ROLIPRAM | C16 H21 N O3 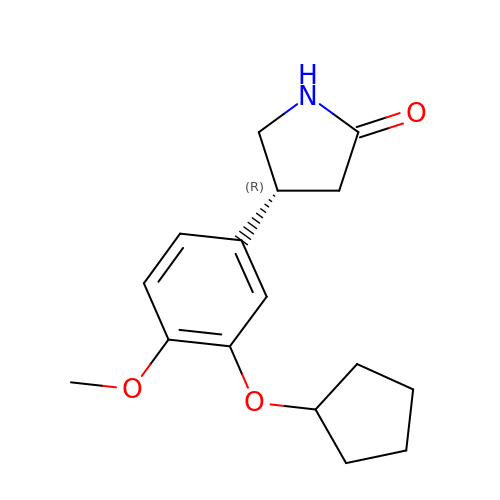| HJORMJIFDVBMOB-LBPRGKRZSA-N>HGDHMHNHDTKMDTMSKDMMSMEKIVVPVQQLDPQNGNKDVGTVEITESAYGLVFTPKLHDLAHGLHGFHIHEKPSCEPKEKDGKLVAGLGAGGHWDPKQTQKHGYPWSDDAHMGDLPALFVMHDGSATTPVLAPRLKKLAEVKGHSLMIHAGGDNHSDHPAPLGGGGPRMAC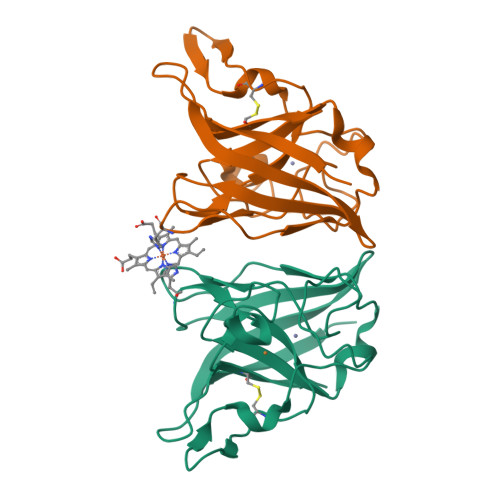GVIK[4x]> IVGGYTCGANTVPYQVSLNSGYHFCGGSLINSQWVVSAAHCYKSGIQVRLGEDNINVVEGNEQFISASKSIVHPSYNSNTLNNDIMLIKLKSAASLNSRVASISLPTSCASAGTQCLISGWGNTKSSGTSYPDVLKCLKAPILSDSSCKSAYPGQITSNMFCAGYLEGGKDSCQGDSGGPVVCSGKL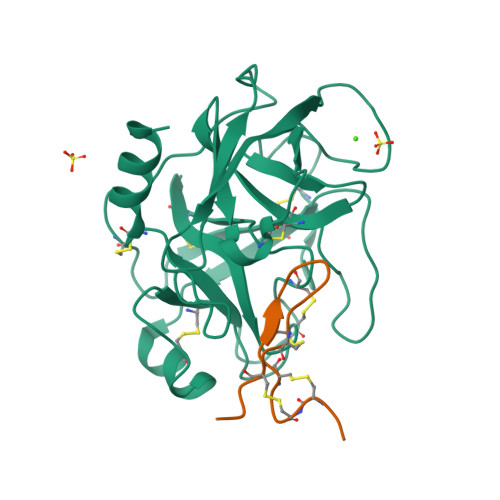QGIVSWGSGCAQKNKPGVYTKVCNYVSWIKQTIASN;> EPCCDSCRCTKSIPPQCHCANI>SMPSETPQAEVGPTGCPHRSGPHSAKGSLEKGSPEDKEAKEPLWIRPDAPSRCTWQLGRPASESPHHHTAPAKSPKILPDILKKIGDTPMVRINKIGKKFGLKCELLAKCEFFNAGGSVKDRISLRMIEDAERDGTLKPGDTIIEPTSGNTGIGLALAAAVRGYRCIIVMPEKMSSEKVDVLRALGAEIVRTPTNARFDSPESHVGVAWRLKNEIPNSHILDQYRNASNPLAHYDTTADEILQQCDGKLDMLVASVGTGGTITGIARKLKEKCPGCRIIGVDPEGSILAEPEELNQTEQTTYEVEGIGYDFIPTVLDRTVVDKWFKSNDEEAFTFARMLIAQEGLLCGGSAGSTVAVAVKAAQELQEGQRCVVILPDSVRNYMTKFLSDRWMLQKGFLKEEDLTEKKPWWWHLRVQELGLSAPLTVLPTITCGHTIEILREKGFDQAPVVDEAGVILGMVTLGNMLSSLLAGKVQPSDQVGKVIYKQFKQIRLTDTLGRLSHILEMDHFALVVHEQIQYHSTGKSSQRQMVFGVVTAIDLLNFVAAQERDQK[10x]

Cystathionine beta-synthase (CBS) is an essential metabolic enzyme across all domains of life for the production of glutathione, cysteine, and hydrogen sulfide. Human CBS adopts a unique multi-domain structure: an N-terminal haem binding domain (residues 38–74), a central PLP-dependent catalytic domain (CD, residues 75–382), and a C-terminal regulatory domain (RD, residues 411–551)5,11,12. The RD adopts the evolutionarily conserved Bateman module, consisting of two tandem CBS motifs (CBS-1 and CBS-2) and a surface-exposed loop (residues 516–525) extending from a CBS-2 motif. Here we show using cryo-electron microscopy that full-length human CBS in the basal and SAM-bound activated states polymerises as filaments mediated by a conserved regulatory domain loop.

We pursued the cryo-EM structure of full-length CBS initially using two constructs: one where an N-terminal His-tag was removed during purification (CBSFL) and one with a permanent C-terminal His-tag (CBSFL-CHis). Micrographs of full-length CBS from both constructs in vitreous ice clearly showed the presence of flexible filaments of varying lengths agreeing with 2D classes. Multiple maps were processed using both helical and single particle reconstruction to resolutions of between 3.9 and 3.0 Å. Both constructs resulted in maps with virtually identical conformations, and both were used for modelling. The CBS filament adopts a left-handed helical architecture with a twist of −108° and a rise of 51 Å. In the basal state, CBS regulatory domains sterically block the catalytic domain active site, resulting in a low-activity filament with three CBS dimers per turn. The domain-swapped dimer, previously observed in crystal structures, is the repeating unit, and helical formation is driven by inter-dimeric RD interactions, i.e., between the RDs of neighbouring subunits of the filament. Here the RD sits atop the active site entrance of the catalytic domain hindering substrate access. Loop 516–525, a β-turn-β extension from the CBS-2 motif in the conserved Bateman module, plays a key role in driving oligomerisation. Though both full-length CBS constructs resulted in highly similar filament maps, one key difference was the observed protein degradation and the presence of slightly shorter oligomers of the CBSFL construct without a permanent His-tag. The CBSΔ516–525 protein, which does not form filaments, is less thermostable than CBSFL by ~5 °C, confirming that filamentation increases stability.WbbB, a lipopolysaccharide O-antigen synthesis enzyme from Raoultella terrigena, contains an N-terminal glycosyltransferase domain with a highly modified architecture that adds a terminal β-Kdo (3-deoxy-d-manno-oct-2-ulosonic acid) residue to the O-antigen saccharide, with retention of stereochemistry. WbbB’s two C-terminal GT domains produce a polymer with a [4)-α-Rhap-(1→3)-β-GlcpNAc-(1→] repeat unit, while the N-terminal domain of the protein contains a GT99 retaining β-Kdo transferase, referred to here as WbbBGT99. Kdo addition blocks further polymerization while creating the epitope recognized by the carbohydrate-binding module of the cognate ABC transporter, allowing export prior to ligation to lipid A-core in the periplasm. The evidence presented above strongly argues that WbbBGT99 is a retaining glycosyltransferase that uses a double-displacement mechanism analogous to that used by retaining glycoside hydrolases.

We determined the structure (at 2.3 Å resolution) of the wild-type enzyme co-crystallized with 5 mM of both CMP and a disaccharide acceptor (α-Rha-(1→3)-β-GlcNAc-C8-methoxybenzamide, 2). Disaccharide density is clearly visible in both active sites, and after building refines with good occupancy (0.9/0.8 and 0.8/0.7 for Rha/GlcNAc in the A and B chains, respectively). The ADP values are similar to those of both the surrounding amino acids and to the Wilson B-factor, indicating that the ligand is well-ordered within its binding site. The acceptor binds to the opposite side of the pocket from Kdo, making interactions exclusively with residues from the N-terminal α/β domain. Glu158 was previously identified as a residue being absolutely required for the reaction, and makes a pair of close hydrogen bonds (both 2.6 Å) to the O3 and O4 hydroxyl groups of rhamnose. Other important hydrogen bonding interactions include O2 to the indole nitrogen of Trp20 and O4 to Arg12, as well as to a structural water molecule. The GlcNAc residue is stacked on Trp54, with the methyl of the acetyl group stacking on Trp20. The amide nitrogen of the GlcNAc points to the indole ring of Trp54, making a strong interaction with the π electrons. Both Trp20 and Trp54 are important for turnover, with Trp54Ala having a larger effect, consistent with its extensive van der Waals contacts with the GlcNAc acceptor residue. The methyl group of the acetyl moiety sits in a well-defined non-polar pocket, with van der Waals contacts with Trp20, Trp54, Leu64, and Ile159.

>[2x]MGLAVFLPPYPFRGLKAPYLWMFYKYLHCATDSILFITGEDYLSVTDDEAQRARWEFDPASMASLGYELPNAQSMACHEYLTLDNAFYETLLSRHHHDPIKSFSAFLTERIPDLETELHALLDSKKGIIDQIDTFISICNCPSLEHVARTLGKEVMHIEIGPLRAPMYRNTAYLDFAGVNGGTEASARYEKCQAEFDIKASLGDLHNYFLEVLPPAEAATHSAAGVVLQVEDDSNLIAYNHDFTNISLLSYVRQRYEKEDILVRAHPGSLFRLRDDVFTIDDSANSLAFINQCNEVFTINSSVGLEAILTGKKTTVLGDCSYAFINELAGASATVNAAAFYLFSYLVPFDLVFNQEYLKFRLGHPEEREIVGKHIEFYSADMPGSLSQAASSLSSLINEAISLEHHHHHH>[3x]HEHNTIPKGASIEVKVQQLDPVNGNKDVGTVTITESNYGLVFTPDLQGLSEGLHGFHIHENPSCEPKEQEGKLTAGLGAGGHWDPKGAKQHGYPWQ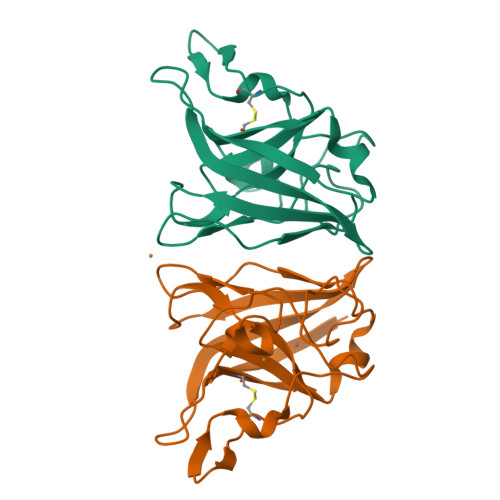DDAHLGDLPALTVLHDGTATNPVLAPRLKHLDDVRGHSIMIHTGGDNHSDHPAPLGGGGPRMACGVIK>[2x]ADNLAEFHVQNQECDSCHTPDGELSNDSLTYENTQCVSCHGTLAEVAETTKHEHYNAHASHFPGEVACTSCHSAHEKSMVYCDSCHSFDFNMPYAKKWLRDEPTIAELAKDKSERQAALASAPHDTVDVVVVGSGGAGFSAAISATDSGAKVILIEKEPVIGGNAKLAAGGMNAAWTDQQKAKKITDSPELMFEDTMKGGQNINDPALVKVLSSHSKDSVDWMTAMGADLTDVGMMGGASVNRAHRPTGGAGVGAHVVQVLYDNAVKRNIDLRMNTRGIEVLKDDKGTVKGILVKGMYKGYYWVKADAVILATGGFAKNNERVAKLDPSLKGFISTNQPGAVGDGLDVAENAGGALKDMQYIQAHPTLSVKGGVMVTEAVRGNGAILVNREGKRFVNEITTYDKASAAILAQTGKSAYLIFDDSVRK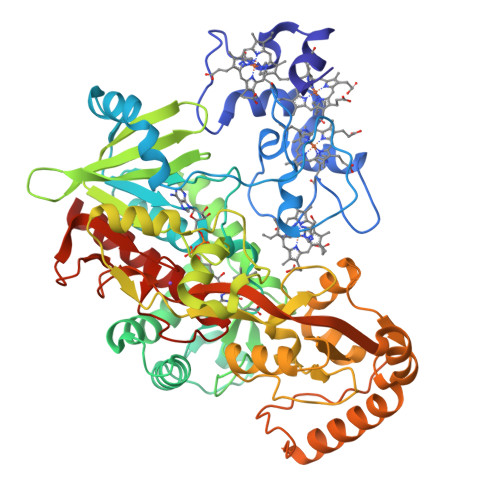SLSKIDKYIGLGVAPTADSLVKLGKMEGIDGKALTETVARYNSLVSSGKDTDFERPNLPRALNEGNYYAIEVTPGVHHTMGGVMIDTKAEVMNAKKQVIPGLYGAGEVTGGVHGANRLGGNAISDIITFGRLAGEEAAKYSKKN> MDPIINGNSANVYLTDSYLKGVISFSECNALGSYIFNGPYLKNDYTNLISRQNPLIEHMNLKKLNITQSLISKYHKGEIKLEEPTYFQSLLMTYKSMTSSEQIATTNLLKKIIRRAIEISDVKVYAILNKLGLKEKDKIKSNNGQDEDNSVITTIIKDDILSAVKDNQSHLKADKNHSTKQKDTIKTTLLKKLMCSMQHPPSWLIHWFNLYTKLNNILTQYRSNEVKNHGFTLIDNQTLSGFQFILNQYGCIVYHKELKRITVTTYNQFLTWKDISLSRLNVCLITWISNCLNTLNKSLGLRCGFNNVILTQLFLYGDCILKLFHNEGFYIIKEVEGFIMSLILNITEEDQFRKRFYNSMLNNITDAANKAQKNLLSRVCHTLLDKTVSDNIINGRWIILLSKFLKLIKLAGDNNLNNLSELYFLFRIFGHPMVDERQAMDAVKINCNETKFYLLSSLSMLRGAFIYRIIKGFVNNYNRWPTLRNAIVLPLRWLTYYKLNTYPSLLELTERDLIVLSGLRFYREFRLPKKVDLEMIINDKAISPPKNLIWTSFPRNYMPSHIQNYIEHEKLKFSESDKSRRVLEYYLRDNKFNECDLYNCVVNQSYLNNPNHVVSLTGKERELSVGRMFAMQPGMFRQVQILAEKMIAENILQFFPESLTRYGDLELQKILELKAGISNKSNRYNDNYNNYISKCSIITDLSKFNQAFRYETSCICSDVLDELHGVQSLFSWLHLTIPHVTIICTYRHAPPYIGDHIVDLNNVDEQSGLYRYHMGGIEGWCQKLWTIEAISLLDLISLKGKFSITALINGDNQSIDISKPIRLMEGQTHAQADYLLALNSLKLLYKEYAGIGHKLKGTETYISRDMQFMSKTIQHNGVYYPASIKKVLRVGPWINTILDDFKVSLESIGSLTQELEYRGESLLCSLIFRNVWLYNQIALQLKNHALCNNKLYLDILKVLKHLKTFFNLDNIDTALTLYMNLPMLFGGGDPNLLYRSFYRRTPDFLTEAIVHSVFILSYYTNHDLKDKLQDLSDDRLNKFLTCIITFDKNPNAEFVTLMRDPQALGSERQAKITSEINRLAVTEVLSTAPNKIFSKSAQHYTTTEIDLNDIMQNIEPTYPHGLRVVYESLPFYKAEKIVNLISGTKSITNILEKTSAIDLTDIDRATEMMRKNITLLIRILPLDCNRDKREILSMENLSITELSKYVRERSWSLSNIVGVTSPSIMYTMDIKYTTSTISSGIIIEKYNVNSLTRGERGPTKPWVGSSTQEKKTMPVYNRQVLTKKQRDQIDLLAKLDWVYASIDNKDEFMEELSIGTLGLTYEKAKKLFPQYLSVNYLHRLTVSSRPCEFPASIPAYRTTNYHFDTSPINRILTEKYGDEDIDIVFQNCISFGLSLMSVVEQFTNVCPNRIILIPKLNEIHLMKPPIFTGDVDIHKLKQVIQKQHMFLPDKISLTQYVELFLSNKTLKSGSHVNSNLILAHKISDYFHNTYILSTNLAGHW;>MEKFAPEFHGEDANNRATKFLESIKGKFTSPKDPKKKDSIISVNSIDIEVTKESPITSNSTIINPTNETDDTAGNKPNYQRKPLVSFKEDPTPSDNPFSKLYKETIETFDNNEEESSYSYEEINDQTNDNITARLDRIDEKLSEILGMLHTLVVASAGPTSARDGIRDAMVGLREEMIEKIRTEALMTNDRLEAMARLRNEESEKMAKDTSDEVSLNPTSEKLNNLLEGNDSDNDLSLEDF[4x]

RSV initiates viral infection by delivering into the host cell a virus-specific RNA synthesis machine required for both genome replication and gene transcription. The catalytic core is a 250 kDa large (L) protein that catalyzes the RNA polymerization in both replication and transcription, the cap addition, and cap methylation of nascent viral mRNAs. A tetrameric phosphoprotein (P) is essential to modulate and constitute an active RNA polymerase with L4,5. Here, we characterize the structure of the RSV polymerase (L:P) using cryo-electron microscopy (cryo-EM).

A total of 2600 movies gave rise to the final 3.67 Å map, refined with 253,372 particles selected from multiple rounds of 2D and 3D classifications. The final atomic model contains the RdRp domain (blue) and the Cap domain (green) of the RSV L protein, and the oligomerization domain (POD, red) and C-terminal domain (PCTD, orange) of tetrameric P proteins (representative model fitting with the map). We have assigned residues to domains as follows: RdRp, 1-945; Cap, 946-1461; POD, 128-157; PCTD, 158-241. The RdRp domain adopts a conventional “fingers-palm-thumb” right-hand fold as many other RNA and DNA polymerases. POD is fully assembled into a four-helix bundle as expected. However, the 3.67 Å cryo-EM map revealed no extra density for the connector domain (CD), the MT domain and the C-terminal domain (CTD) of L as well as the N-terminal domain (NTD) of P. We speculate that the missing density of L is due to significant structural rearrangements of L, and the missing density of P is primarily due to the intrinsic flexibility of P. The interactions between L and a tetrameric P can be divided into three parts: (1) two of four-helix bundles of POD and the RdRp; (2) two flexible PCTD chains wrap around the surface of RdRp and stabilize the base of the tetrameric POD; (3) one flexible PCTD chain extends to the positively charged “palm” motif of RdRp and the edge of the putative NTP entrance channel. Interestingly, four chains of PCTD adopt four different conformations and interact broadly with the RdRp domain of L. However, the nonsymmetric structures of PCTD suggest that P likely plays a nonsymmetric structural role more than previously appreciated.>MHHHHHHSSGRENLYFQGMNMEITNLKSYKELVTLSAEEKTKDLKDYLNDKNRSESLIKKFKNFYMDLSRQRYSEKTLNKLVEYAEEVELKKKVEKTFMGEKVNMTENRSVLHTALRIPIEKINTHKIIIDNKNVLEDVHGVLKKIEKYSDDIRNGVIKTCKNTKFKNVICIGIGGSYLGTEFVYEAMKYYYYNMELNKNEKDQVNNFNNNYDQDNVFNVRFLANVDPNDVNRAIQNLDQYDTLVIIISKTFTTAETMLNARSIKKWLSLKIKDDENLSKHMVAVSTNLKLTDEFGISRDNVFEFWDWVGGRFSVTSSVGILPLSIAFGYKNMRNFLNGCHDMDEHFLHADLKENIPVLLALTSFYNSHFFDYKNVAILPYFQNLLKFSAHIQQLSMESNGKSVDRNNQPIHYNTCQVYFGEPGTNGQHSFYQLIHQGQVIPVELIGFKHSHFPIKFDKEVVSNHDELMTNFFAQADALAIGKTYEQVKEENEKNKMSPELLTHKVFNGNRPSTLLLFDELNFYTCGLLLSLYESRIVAEGFLLNINSFDQWGVELGKVLAKEVRNYFNDTRNQKKSDNT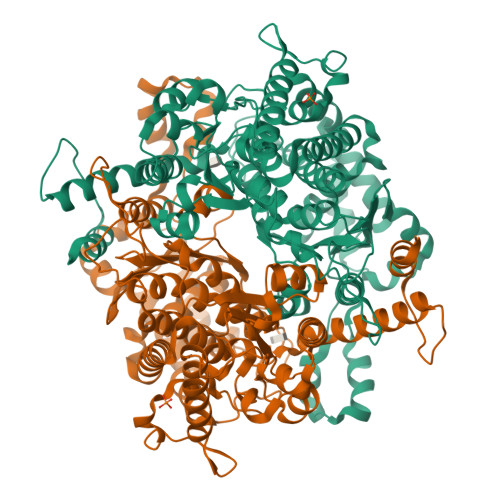YNFNESTKILLNYYLSK[2x]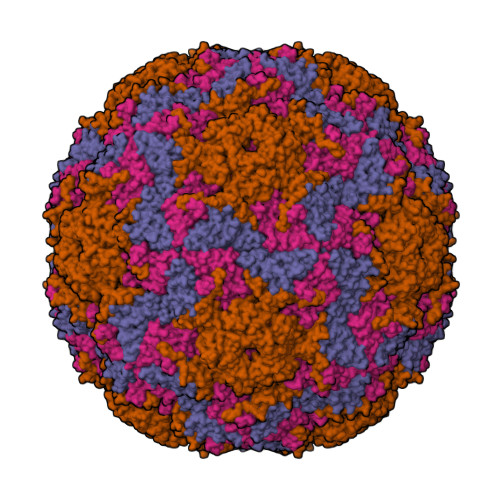> GDPIADMIDQTVNNQVNRSLTALQVLPTAANTEASSHRLGTGVVPALQAAETGASSNASDKNLIETRCVLNHHSTQETAIGNFFSRAGLVSIITMPTTDTQNTDGYVNWDIDLMGYAQLRRKCELFTYMRFDAEFTFVVAKPNGVLVPQLLQYMYVPPGAPKPTSRDSFAWQTATNPSVFVKMTDPPAQVSVPFMSPASAYQWFYDGYPTFGEHLQANDLDYGQCPNNMMGTFSIRTVGTEKSPHSITLRVYMRIKHVRAWIPRPLRNQPYLFKTNPNYKGNDIKCTSTSRDKITTL;> SPSAEACGYSDRVAQLTIGNSTITTQEAANIVIAYGEWPEYCPDTDATAVDKPTRPDVSVNRFFTLDTKSWAKDSKGWYWKFPDVLTEVGVFGQNAQFHYLYRSGFCVHVQCNASKFHQGALLVAVLPEYVLGTIAGGTGNENSHPPYATTQPGQVGAVLTHPYVLDAGIPLSQLTVCPHQWINLRTNNCATIIVPYMNTVPFDSALNHCNFGLLVIPVVPLDFNAGATSEIPITVTIAPMCAEFAGLRQAVKQ;> GIPTELKPGTNQFLTTDDGVSAPILPGFHPTPPIHIPGEVHNLLEICRVETILEVNNLKTNETTPMQRLCFPVSVQSKTGELCAAFRADPGRDGPWQSTILGQLCRYYTQWSGSLEVTFMFAGSFMATGKMLIAYTPPGGNVPADRITAMLGTHVIWDFGLQSSVTLVVPWISNTHYRAHARAGYFDYYTTGIITIWYQTNYVVPIGAPTTAYIVALAAAQDNFTMKLCKDTEDIEQTANIQ;> MGSQVSTQRSGSHENSNSASEGSTINYTTINYYKDAYAASAGRQDMSQDPKKFTDPVMDVIHEMAPPLK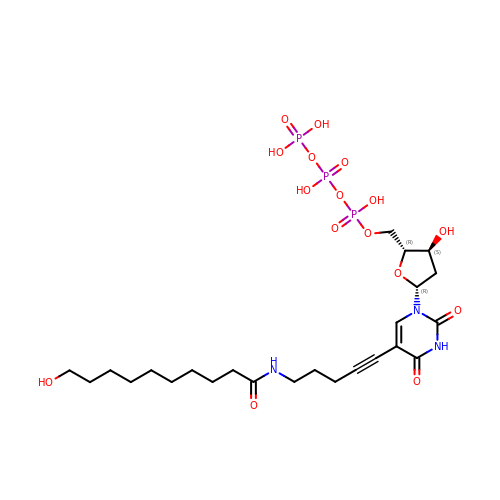2'-deoxy-5-{5-[(10-hydroxydecanoyl)amino]pent-1-yn-1-yl}uridine 5'-(tetrahydrogen triphosphate) | C24 H40 N3 O16 P3 | UGHLPDROZCTFGX-TUNNFDKTSA-N> NLYQFGRMIWNRTGKLPILSYGSYGCYCGWGGQGPPKDATDRCCLVHDCCYTRVGDCSPKMTLYSYRFENGDIICDNKDPCKRAVCECDREAAICLGENVNTYDKKYKSYEDC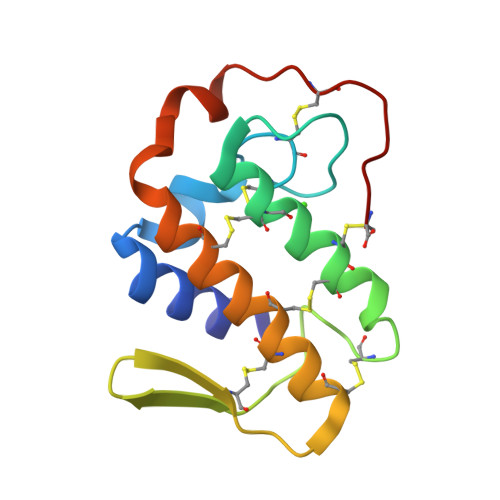TEEVQEC>[3x]MSNLDELASSRQTVLEPQDEVRIVGQYYDDKTAKLVRKYGPGPRIHYHVGYYPSSEAPRHTRDVTPDAFRRSIRLHQEGLLRYAAKIWGAEHRLSGRILDVGCGLGGGSLFWAQEYGADVTAVTNAPEHAPIVEGFARECGVGGR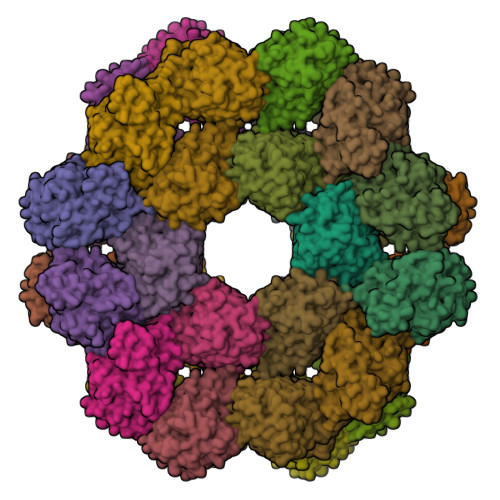VRTLVCDAMHLPLDGGPYDAAVAIESSGYFDRPVWFERLAHVLRPGGSVCIEEVFTTRPHGADVWAEYFYTKPATVLDYAEAAKAAGFELVDDVDATSETLPFWEESTAWTKAVLDSDSTLSAVDRRQLRISLMANQALGAEWQAGGLRLGFLRFERK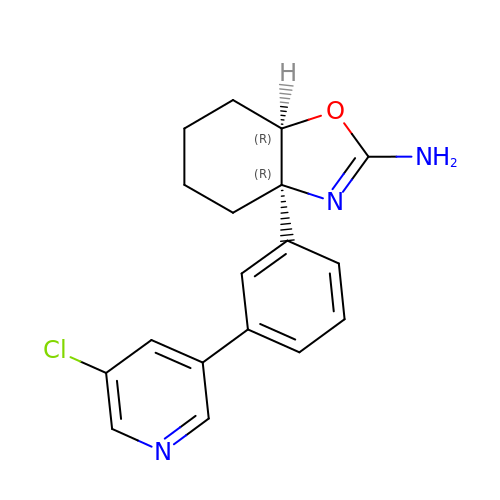(3aR,7aR)-3a-[3-(5-chloropyridin-3-yl)phenyl]-3a,4,5,6,7,7a-hexahydro-1,3-benzoxazol-2-amine | C18 H18 Cl N3 O | NVRCQOQFKIFZLP-SJLPKXTDSA-N> GSQPEQKTLSLPGTYRHVDRTTGQVLTCDKCPAGTYVSEHCTNMSLRVCSSCPAGTFTRHENGIERCHDCSQPCPWPMIERLPCAALTDRECICPPGMYQSNGTCAPHTVCPVGWGVRKKGTENEDVRCKQCARGTFSDVPSSVMKCKAHTDCLGQNLEVVKPGTKETDNVCGMRLFFSSTASGR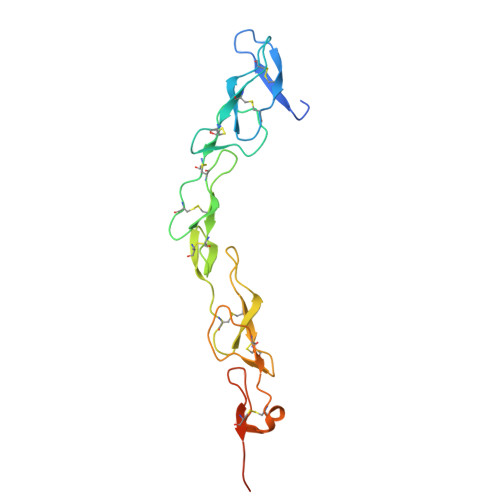GLVPR> MSLGAKPFGEKKFIEIKGRRMAYIDEGTGDPILFQHGNPTSSYLWRNIMPHCAGLGRLIACDLIGMGDSDKLDPSGPERYAYAEHRDYLDALWEALDLGDRVVLVVHDWGSALGFDWARRHR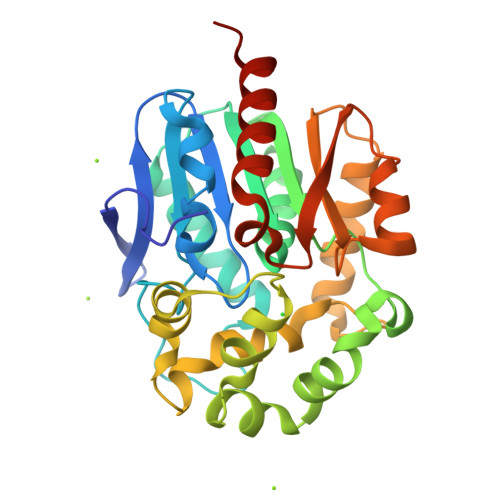ERVQGIAYMEAIAMPIEWADFPEQCRDLFQAFRSQAGEELVLQDNVFVEQVLPGCILRPLSEAEMAAYREPFLAAGEARRPTLSWPRQIPIAGTPADVVAIARDYAGWLSESPIPKLFINAEPGALTTGRMRDFCRTWPNQTEITVAGAHFIQEDSPDEIGAAIAAFVRRLRPAHHHHHH> PTIFEERHLKYISQLGKGNFGSVELCRYDPLGDNTGALVAVKQLQHSGPDQQRDFQREIQILKALHSDFIVKYRGVSYGPGRPELRLVMEYLPSGCLRDFLQ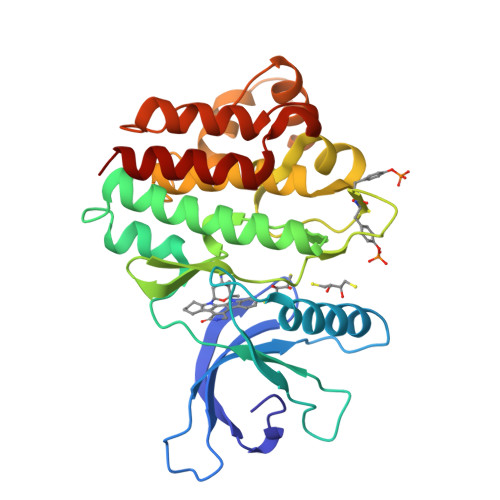RHRARLDASRLLLYSSQICKGMEYLGSRRCVHRDLAARNILVESEAHVKIADFGLAKLLPLDKDYYVVREPGQSPIFWYAPESLSDNIFSRQSDVWSFGVVLYELFTYCDKSCSPSAEFLRMMGCERDVPALCRLLELLEEGQRLPAPPACPAEVHELMKLCWAPSPQDRPSFSALGPQLDMLWSGSR> PIPTAPRENSLMFLSTLPDDTVPAYGNVRTPPVNYLPGEITDLLQLARIPTLMAFERVPEPVPASDTYVPYVAVPTQFDDRPLISFPITLSDPVYQNTLVGAISSNFANYRGCIQITLTFCGPMMARGKFLLSYSPPNGTQPQTLSEAMQCTYSIWDIGLNSSWTFVVPYISPSDYRETRAITNSVYSA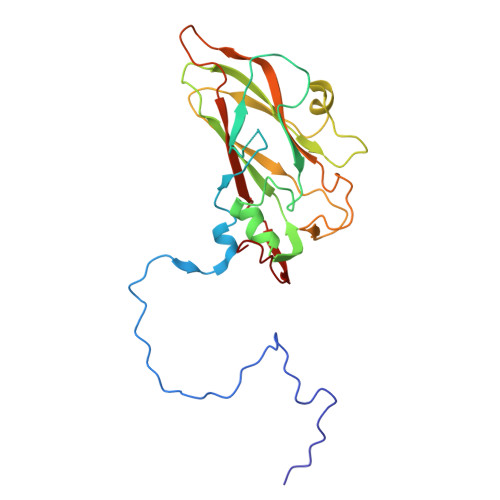DGWFSLHKLTKITLPPDCPQSPCILFFASAGEDYTLRLPVDCNPSYVF> MNHKVHHH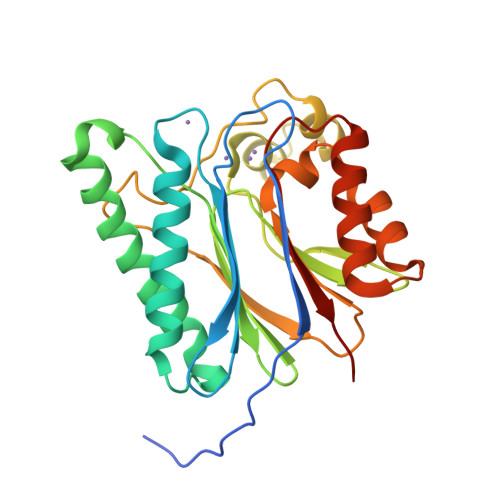HHHIEGRHMELGTMLEAQFFTDTGQHRDKNEDAGGIFYNQTNQQLLVLCDGMGGHKAGEVASKFVTDELKSRFEAENLIEQHQAENWLRNNIKDINFQLYHYAQENAEYKGMGTTCVCALVFEKSVVIANVGDSRAYVINSRQIEQITSDHSFVNHLVLTGQITPEEAFTHPQRNIITKVMGTDKRVSPDLFIKRLNFYDYLLLNSDGLTDYVKDNEIKRLLVKEGTIEDHGDQLMQLALDNHSKDNVTFILAAIEGDKV> ALWQFNGMIKCKIPSSEPLLDFNNYGCYCGLGGSGTPVDDLDRCCQTHNNCYKQAKKLDSCKVLVDNPYTNNYSYSC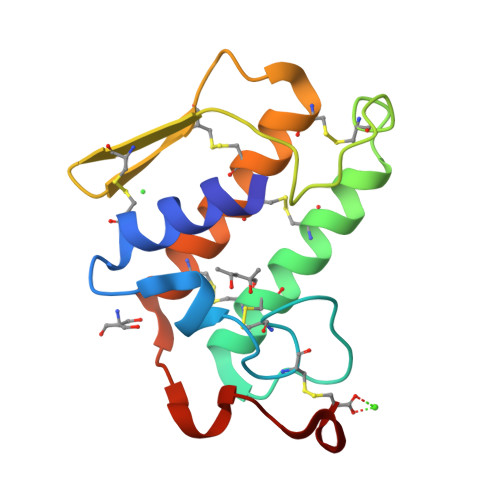SNNEITCSSENNACEAFICNCDRNAAICFSKVPYNKEHKNLDKKNC> MSNIQNMSLEDIMGERFGRYSKYIIQDRALPDIRDGLKPVQRRILYSMNKDSNTFDKSYRKSAKSVGNIMGNFHPHGDSSIYDAMVRMSQNWKNREILVEMHGNNGSMDGDPPAAMRYTEARLSEIAGYLLQDIEKKTVPFAWNFDDTEKEPTVLPAAFPNLLVNGSTGISAGYATDIPPHNLAEVIDAAVYMIDHPTAKIDKLMEFLPGPDFPTGAIIQGRDEIKKAYETGKGRVVVRSKTEIEKLKGGKEQIVITEIPYEINKANLVKKIDDVRVNNKVAGIAEVRDESDRDGLRIAIELKKDANTELVLNYLFKYTDLQINYNFNMVAIDNFTPRQVGIVPILSSYIAHRREVILARSRFDKEKAEKRLHIVEGLIRVISILDEVIALIRASENKADAKENLKVSYDFTEEQAEAIVTLQLYRLTNTDVVVLQEEEAELREKIAMLAAIIGDERTMYNLMKKELREVKKKFATPRLSSLEDTAKALEHHHH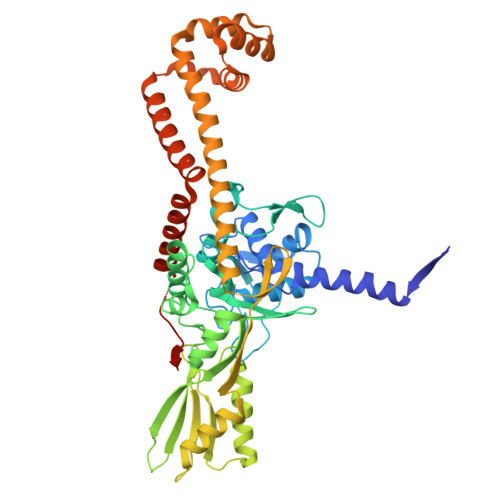HH>[4x]GITGTWYNQLGSTFIVTAGADGALTGTYESAVGNAES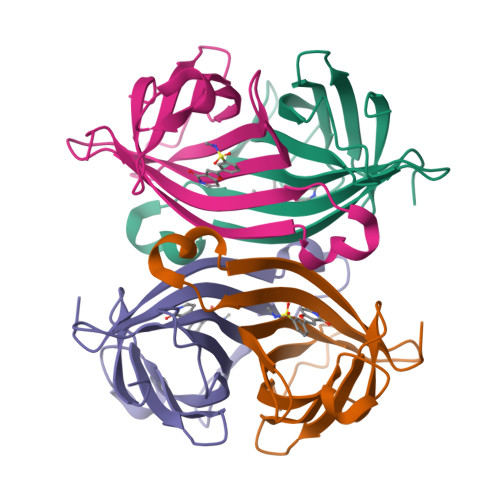RYVLTGRYDSAPATDGSGTALGWTVAWKNNYRNAHSATTWSGQYVGGAEARINTQWLLTSGTTEANAWKSTLVGHDTFTKVKP> SNAMLLYTKKDDIYSDIVRMILLIKGA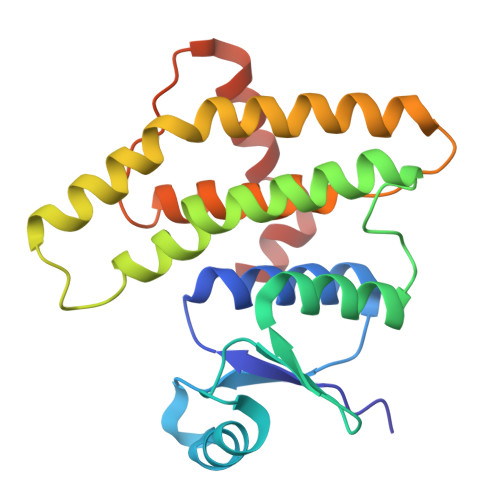NAKIVDVSKEENSKHLEELNIITPNGNIPTLSTDDFAVYRLSVIIEAIEDLYPFPPMFPVFPKQRANARILLEYVNKTFLQNIIKLQSPDLDEKQANEIKMLMQRDIISTYKKIVSEREVNAESNPDAQNINVLTLIITFVFYYFIKLKISIPTKDKNIIKEIKELLSEPNFIKTIK4-amino-1-beta-D-glucopyranosylpyrimidin-2(1H)-one | C10 H15 N3 O6 | 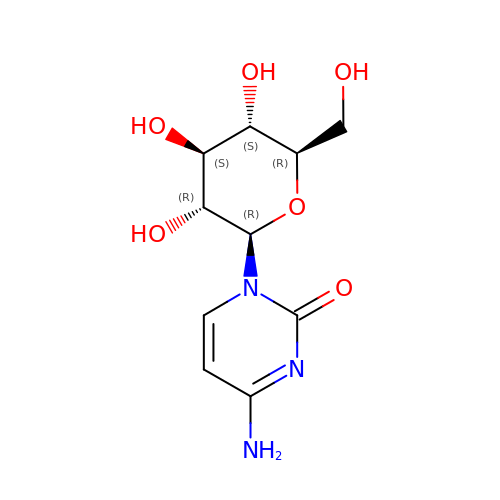YYUQXKHCNLFJNF-DDIGBBAMSA-N>SNAMIFPKQYPIINFTTAGATVQSYTNFIRAVRGRLTTGADVRHEIPVLPNRVGLPINQRFILVELSNHAELSVTLALDVTNAYVVGYRAGNSAYFFHPDNQEDAEAITHLFTDVQNRYTFAFGGNYDRLEQLAGNLRENIELGNGPLEEAISALYYYSTGGTQLPTLARSFIICIQMISEAARFQYIEGEMRTRIRYNRRSAPDPSVITLENSWGRLSTAIQESNQGAFASPIQLQRRNGSKFSVYDVSILIPIIALMVYRCAPPPSSQF[2x]

Ricin contains an active A subunit (RTA) and a B subunit (RTB), which promotes retrograde transport into the endoplasmic reticulum (ER). RTA and Stx2A1 are ribosome inactivating proteins (RIPs), which remove a highly conserved adenine base (A4324 in rat) from the sarcin/ricin loop (SRL) of the 28S rRNA, leading to the inhibition of translation, ribotoxic stress, and apoptosis. We showed that RTA is recruited to the SRL by binding first to a conserved sequence at the C-terminal domain (CTD) of ribosomal P-stalk proteins. The X-ray crystal structure analysis showed that RTA binds the last six amino acids of P11 in a hydrophobic pocket at its CTD.

The RTA-RU-NT-202, RTA-RU-NT-165, and RTA-RU-NT-192 structures were all determined at 1.8 Å. The RTA-RU-NT-165 and RTA-RU-NT-192 structures were determined in the monoclinic P21 space group with the RTA-RU-NT-202 complex structures solved in the orthorhombic P212121 space group. After superimposing these structures and the structure of RTA with RU-NT-206 (38), the RMSD values range from 0.23 to 0.46 Å, demonstrating no significant conformational changes in the RTA backbone upon binding of these inhibitors. Both RU-NT-165 and RU-NT-192 exhibited more comparable binding patterns, where the carboxylate group within the thiophene ring of each inhibitor formed a salt bridge with the Arg234 side chain and a hydrogen bond with the main chain amide nitrogen of Arg235. Moreover, the ethyl groups at the 2-position within the benzene rings from RU-NT-165 and RU-NT-192 formed distinct hydrophobic interactions with Leu207. The fluorine atom of the fluorobenzene ring in RU-NT-202 uniquely interacted with Val242 in RTA, while making closer contacts with Ile247 and Leu248. Additionally, in the RTA-RU-NT-165 and RTA-RU-NT-192 structures, the carboxylate group from one of the inhibitors formed a spurious salt bridge with Arg234 from the second RTA copy within the asymmetric unit. In RU-NT-165, the carboxylate being nearly coplanar with the thiophene spreads the charge across both the thiophene and the carboxylate, potentially reducing the ionic interactions with both Arg234 and Arg235 compared to RU-NT-192. In contrast, RU-NT-165 has a nearly coplanar orientation between the thiophene ring and carboxylate group, which diminishes the relative strength of its noncovalent interactions with Arg234 and Arg235 compared to RU-NT-192. RU-NT-192 demonstrated a 2-fold improvement in the Ki value compared to RU-NT-165 and a 4-fold improvement in the Ki value compared to RU-NT-202. RU-NT-165 improved the EC50 by 5-, 12.5-, and >500-fold at 125, 250, and 500 μM, respectively, relative to ricin alone with no compound. RU-NT-165 had an EC50 value of 50 pM at 250 μM.> MAHAGRTGYDNREIVMKYIHYKLSQRGYEWDAGDDVEENRTEAPEGTESEVVHLTLRQAGDDFSRRYRRDFAEMSSQLHLTPFTARGRFATVVEELFRDGVNWGRIVAFF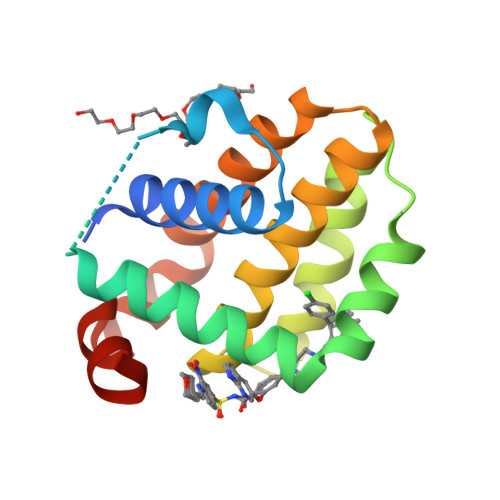EFGGVMCVESVNREMSPLVDNIALWMTEYLNRHLHTWIQDNGGWDAFVELYGPSMR>MKEQQKAIFIENIKSTCAVDEQMAKELADSLLEIHQLNTGVNEQTLINEVFLTKFALYLKIGKEVALDWVRKNKDLDTPFPSNTVENQPAQDAKKPVENKVQVYGAMTVGSSPVNKTLNRLTNDLLKEVVERGKTQKAQKLRAYIFDQLARRLEASLSQEQINDLYNRIRGTGDYTKSESFSEEQLKILKEKVVPELKRELSDLSNGNVNILGLDVSREDKYAFDTTNIFSVWFSNNPAVYMPQHVKTQVEKTAKLNQPGKTRIVFSSLCLNETAQIDFQQWAKENNIELVDIDSIDLKSVSETDAQLLNLAKDELGAMRKGKGGNPAAASDLVRWVDVIIGESSTYIDIDLPMNDKKVTVEVHSGFPVLLNMGSALTKDGQQPAMENPAFNTDMIAYSKDKEARRQIIEGVAKKIIARYENCAKYIEESKNEELVRLKNSPGYKLFVEKTDGKFDLCTLRAAVSEAHQDALSFATFFGAEYFAKTFATQELIPVIKEAIQHQNQDLLTSVIENHIEKQHLNDYPKTPDGIKKLLKSFQGIVYKPLVMEFSGPSAVSSSWVEAISGRSIPRNFEYLAEPMSQPLRVLQHYACVSGKANFSSDNIPKWCELQSDVEKRQQQREDGLSWLPDAQEKLKREGQQAKLEEEQRIKLEEEQRIKLEEEQRIKLEEEQRIKLEEEQRIKLEEEQRIKLEEEQRIKLEEEQRIKLEEEQRIKLEEEHKSKKYFAQSD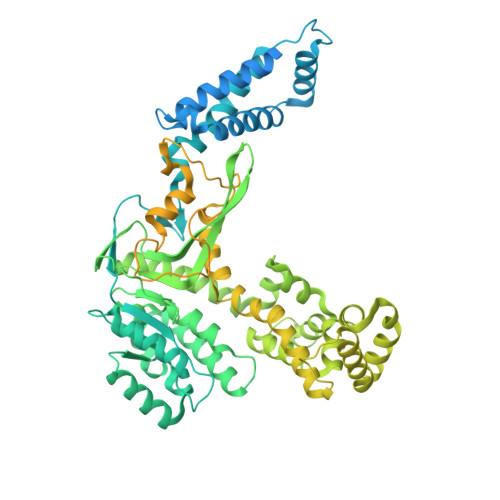AIDLILNNFENEINSIGAYYAPAKQRAIELLDTLRKYKEEAFNDPSREKLISFAQSTKRAIQEATPILQKDLGWGDYLTNLAKQLVNAVTFAVAYAVTFGTTGHQGFFALKSSLAVSQSQNLEGAINSELSQKNC[4x]>[8x]MVRIAVAGAAGRMGRNLVKAAHHNPVAKVAAGSERPESSLVGVDLGELCGEGKFDVV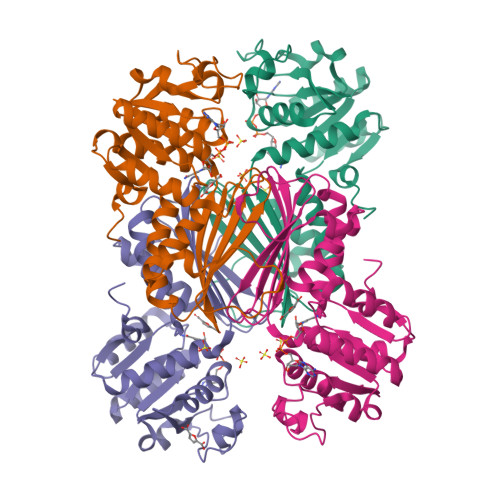VCDDLAKQIDQFDVIIDFTAPASTLNNLALCQQYGKSIVIGTTGFTEEQREQIDLVAQQVPVVMAPNYSVGVNLVFKLLEKAAKVMGDYCDIEIVEAHHRHKVDAPSGTAIGMGEAIAGAMGNKLSDVAVYAREGITGERTKDEIGFATIRAGDIVGEHTAMFADIGERVEITHKATDRMTFANGAVKAAVWLHEKPAGFYTMTDVLGLNDL> K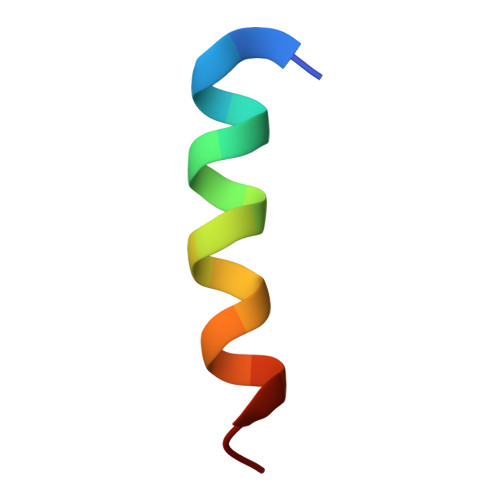TSAAAQLDELMAHLTEMQ> ALRIDYPAALQILMEGGTHMVCTGRTHTDRICRFKWLCYSNEAEEFIFFHGNTSVMLPNLGSRRFQPALLDLSTVEDHNTQYFNFVELPAAALRFMPKPVFVPDVALIANRFNPDNLMHVFHDDLLPLFYTLRQFPGLAHEARLFFMEGWGEGAHFDLYKLLSPKQPLLRAQLKTLGRLLCFSHAFVGLSKITTWYQYGFVQPQGPKANILVSGNEIRQFARFMTEKLNASHTGVPLAAEYILVFARTQNRLILNEAELLAALAQEFQMKTVTVSLEDHTFADVVRLVSNASMLVSMHGAQLVTTLFLPRGATVVELFPYAVNPDHYTPYKTLAMLPGMDLQYVAWRNMMPENTVTHPERPWDQGGITHLDRAEQARILSSREVPRHLCCRNPEWLFRIYQDTKVDIPSLIQTIRRVVAGAPGPRKQKWTAGLYPGKVREARCQASVHGASEARLTVSWQIPWNLKYLKVAEVKYEVWLQEAGENTYVPYILALQNHTFTENIKP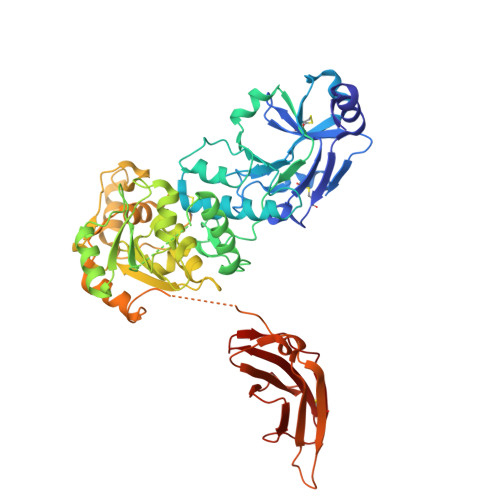FTTYLVWVRCIFNKILLGPFADVLVCNT>GHMRRVVITGLGIVSCLGNDKDTVSANLRAGRPGIRFNPSYAEMGLRSHVSGSVDLNLEELIDRKVFRFMGDAAAYAYLAMEQAIKDSGLTPEQISNPRTGLIAGSGGASTLNQMEAIDTLREKGVKRIGPYRVTRTMGSTVSACLATPFQIKGVNYSISSAAATSAHCIGQAMEQIQLGKQDVVFAGGGEEEHWSQSCLFDAMGALSTQYNETPEKASRAYDAKRDGFVIAGGGGMVVVEELEHALKRGAKIYAEIVGYGATSDGYDMVAPSGEGAIRCMQQALATVDAPIDYLNTHGTSTPVGDVAEIRGVREVFGDKAPAISSTKSLSGHSLGAAGVHEAIYCLLMMEGGFIAGSANIDELDPEVADLPILRETRENAKLDTVMSNSFGFGGTNATLVLKRWQG[2x]

Background: FabB (3-oxoacyl-[acyl-carrier-protein] synthase 1) is part of the fatty acid synthesis II pathway found in bacteria and a potential target for antibiotics. The enzyme catalyses the Claisen condensation of malonyl-ACP (acyl carrier protein) with acyl-ACP via an acyl-enzyme intermediate. Cells lacking FabB are auxotroph for unsaturated fatty acids, making FabB an essential gene for the bacteria.

12 Here, we report the crystal structure of an intermediate-mimicking PaFabB variant at 1.3 Å resolution. Here, the catalytic residue Cys161 of PaFabB was mutated to Ala161. In the Ala variant, the presumably negatively charged Cys in the w. t. form is replaced with a neutral residue, thus mimicking more closely the charge of the lauryl intermediate. PaFabB C161A crystallized as a dimer and has the same overall fold as observed before for FabB and FabF from other organisms. The crystal was in the space group C 2 2 21 and contained 2 protein molecules in the asymmetric unit. The two catalytic histidines, His296 and His331, are highly conserved and well aligned with the catalytic histidines from both VcFabB and PaFabF. Due to the high concentration of ethylene glycol (20% v/v) and salt in the well and protein buffers, respectively (150 mM NaCl and 200 mM NaI), 18 ethylene glycol molecules and 11 ions (Cl - and I -) were identified and placed in the crystal structure of PaFabB C161A during refinement. Some of these molecules were found to bind in the active site of the protein. As can be seen from the crystal structure, Phe391 adopts the ‘open’ conformation as expected for an intermediate-mimicking FabB variant (dihedral angle C-CA-CB-CG = 170.2 o). The C161A mutation of FabB in this crystal structure causes Phe 391 to be in the ‘open’ conformation and allows targeting of the intermediate-acylated state of FabB; in a similar manner to the natural antibiotic platensimycin.N-[(1Z)-2-phenylethanimidoyl]-5-thio-alpha-D-mannopyranosylamine | C14 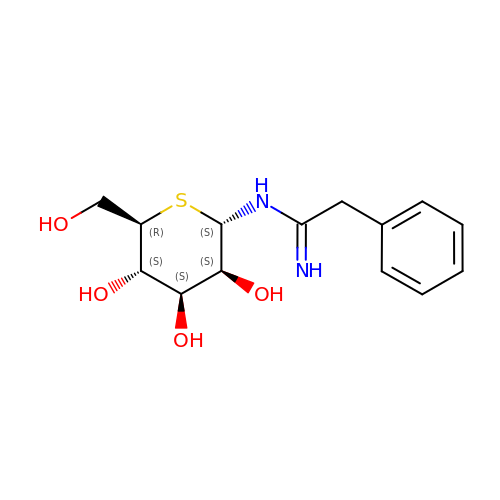H20 N2 O4 S | WKJQYOUTPMBFSL-CYDRSHDDSA-N>MAKRVNTCKCVATPQEKIEYKTKVSRNSNMSKLQAGYLFPEIARRRSAHLLKYPDAQVISLGIGDTTEPIPEVITSAMAKKAHELSTIEGYSGYGAEQGAKPLRAAIAKTFYGGLGIGDDDVFVSDGAKCDISRLQVMFGSNVTIAVQDPSYPAYVDSSVIMGQTGQFNTDVQKYGNIEYMRCTPENGFFPDLSTVGRTDIIFFCSPNNPTGAAATREQLTQLVEFAKKNGSIIVYDSAYAMYMSDDNPRSIFEIPGAEEVAMETASFSKYAGFTGVRLGW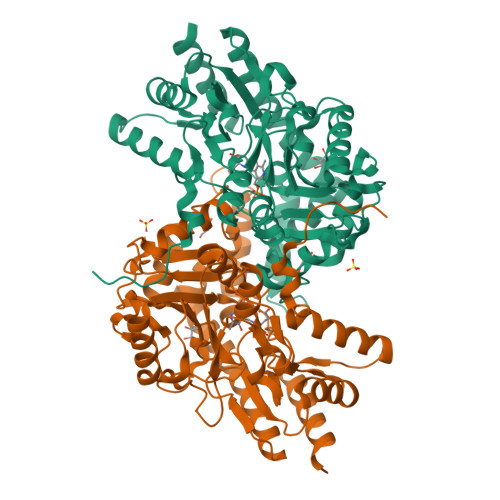TVIPKKLLYSDGFPVAKDFNRIICTCFNGASNISQAGALACLTPEGLEAMHKVIGFYKENTNIIIDTFTSLGYDVYGGKNAPYVWVHFPNQSSWDVFAEILEKTHVVTTPGSGFGPGGEGFVRVSAFGHRENILEACRRFKQLYKHHHHHH[2x]α-Methylacyl-CoA racemase (AMACR; P504S) enzyme plays a vital role in branched-chain fatty acid metabolism by catalyzing the conversion of 2-methyl-branched fatty acyl-CoAs into a near 1 to 1 mixture of the (2R)- and (2S)-epimers, enabling further metabolism. α-Methylacyl-CoA racemase from Mycobacterium tuberculosis (MCR) has been explored as a model to understand the AMACR racemization mechanism and as a drug target. The catalytically active enzyme is a homodimer (with an apparent molecular weight of 83.6 or 89 kDa) with the active site at the interface between the two subunits with catalytic bases contributed by both subunits. Each MCR homodimer contains two active sites formed by residues from the large domain of one subunit and the small domain of the other. Key catalytic residues from the large domain include Asp156 (helix 6) and His126 (helix 5), while Glu241 (beginning of helix 9) is contributed by the small domain.

The ibuprofenoyl-CoA 1 side group is a phenyl ring (C33, C34, C5, C6, C7, C8) with terminal carbons (C4, C3, C2, C1) at the C5 position. Here, the density completely covered the Cα-ring and extended to some of the terminal carbons in most active sites. The terminal carbons showed variability in their orientation. Clear electron density for the thioester carbonyl and Cα-Me groups in the ibuprofenoyl-CoA 1 and S-2-methyldecanoyl-CoA 6 complexes shows a cis conformation. The thioester oxygen forms hydrogen bonds with Asp127, Asp156, and His126. Ibuprofenoyl-CoA 1 and analogs and 2-methyldecanoyl-CoA 6 were relatively potent inhibitors, with ibuprofenoyl-CoA 1 displaying the highest levels of potency (pIC50 = 5.05 ± 0.05; mean ± SEM, n = 3). This level of potency is ∼20-fold less than the corresponding values for human AMACR, where ibuprofenoyl-CoA 1 and analogs had an IC50 value of 200 to 500 nM (pIC50 = 6.7–6.30, respectively). As expected, all these acyl-CoAs were reversible inhibitors and caused competitive inhibition with a Ki value of 3.04 ± 0.34 μM (mean ± SEM, n = 3). In contrast, ibuprofenoyl-CoA 1 is the most potent inhibitor of MCR, and greater variation in inhibition is observed between the other compounds. Our results are consistent with a different mechanism in which the side-chain is held in a relatively static position with the different stereochemical configurations accommodated by a subtle clockwise or anticlockwise rotation of the α-carbon.

>MAGPLSGLRVVELAGIGPGPHAAMILGDLGADVVRIDRPSSVDGISRDAMLRNRRIVTADLKSDQGLELALKLIAKADVLIEGYRPGVTERLGLGPEECAKVNDRLIYARMTGWGQTGPRSQQAGHDINYISLNGILHAIGRGDERPVPPLNLVGDFGGGSMFLLVGILAALWERQSSGKGQVVDAAMVDGSSVLIQMMWAMRATGMWTDTRGANMLDGGAPYYDTYECADGRYVAVGAIEPQFYAAMLAGLGLDAAELPPQNDRARWPELRALLTEAFASHDRDHWGAVFANSDACVTPVLAFGEVHNEPHIIERNTFYEANGGWQPMPAPRFSRTASSQPRPPAATIDIEAVLTDWDGGSGC[12x]>GGCUAGCUGGAGGGGCGCCAGUUCGCUGGUGGUUGGGUGCGGUCGGCUAGCC[2x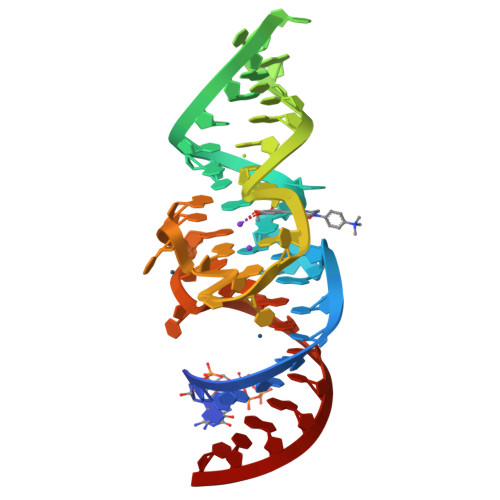]>MQSVELPETHQMLLQTCRDFAEKELFPIAAQVDKEHLFPAAQVKKMGGLGLLAMDVPEELGGAGLDYLAYAIAMEEISRGCASTGVIMSVNNSLYLGPILKFGSKEQKQAWVTPFTSGDKIGCFALSEPGNGSDAGAASTTARAEGDSWVLNGTKAWITNAWEASAAVVFASTDRALQNKSISAFLVPMPTPGLTLGKKEDKLGIRGSSTANLIFEDCRIPKDSILGEPGMGFKIAMQTLDMGRIGIASQALGIAQTALDCAVNYAENRMAFGAPLTKLQVIQFKLADMALALESARLLTWRAAMLKDNKKPFIKE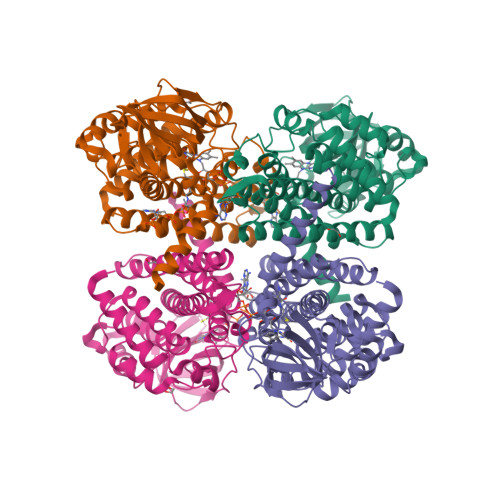AAMAKLAASEAATAISHQAIQILGGMGYVTEMPAERHYRDARITEIYEGTSEIQRLVIAGHLLRSYRSAENLYFQ[8x]> MIKVEIKPSQA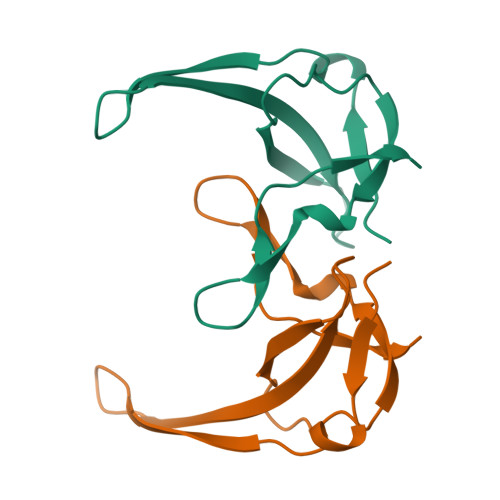QFTTRSGVSRQGKPYSLNEQLCYVDLGNEYPVLVKLTLDEGQPAYAPGLYTVHLSSFKVGQFGSLMIDRLRLVPAK> ANPLYQKHIISINDLSRDDLNLVLATAAKLKANPQPELLKHKVIASCFFEASTRTRLSFETSMHRLGASVVGFSDSANTSLGKKGETLADTISVISTYVDAIVMRHPQEGAARLATEFSGNVPVLNAGDGSNQHPTQTLLDLFTIQETQGRLDNLHVAMVGDLKYGRTVHSLTQA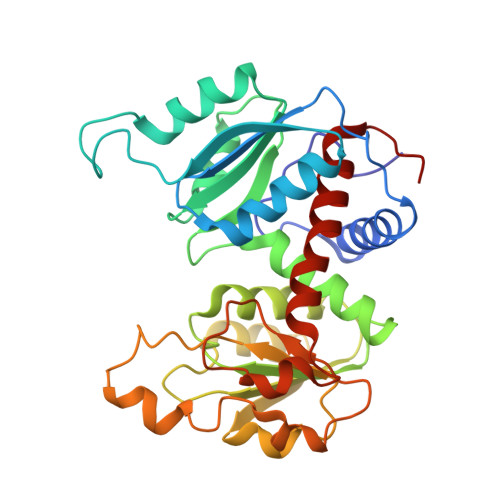LAKFDGNRFYFIAPDALAMPQYILDMLDEKGIAWSLHSSIEEVMAEVDILYMTRVQKERLDPSEYANVKAQFVLRASDLHNAKANMKVLHPLARVDEIATDVDKTPHAWYFQQAGNGIFARQALLALVLNRDLVL>[4x]MTITLTENKRK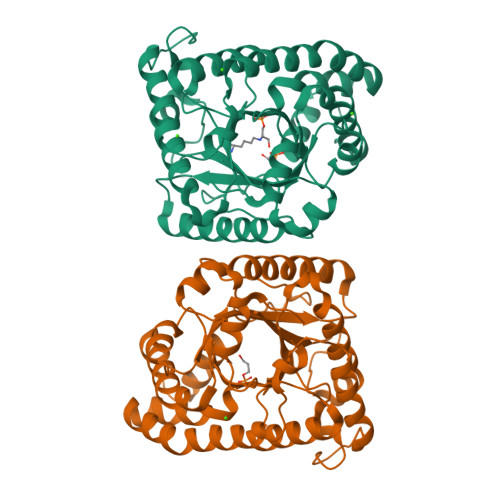SMEKLSVDGVISALAFDQRGALKRMMAQHQTKEPTVEQIEELKSLVSEELTPFASSILLDPEYGLPASRVRSEEAGLLLAYEKTGYDATTTSRLPDCLDVWSAKRIKEAGAEAVKFLLYYDIDGDQDVNEQKKAYIERIGSECRAEDIPFYLEILTYDEKIADNASPEFAKVKAHKVNEAMKVFSKERFGVDVLKVEVPVNMKFVEGFADGEVLFTKEEAAQAFRDQEASTDLPYIYLSAGVSAKLFQDTLVFAAESGAKFNGVLCGRATWAGSVKVYIEEGPQAAREWLRTEGFKNIDELNKVLDKTASPWTEKM>GSMALERTFSIIKPDAVKRNLIGEIYHRIEKAGLQIIAAKMVHLSEEQASGFYAEHEGKPFFEPLKEFMTSGPIMVQVLEGENAIARYRELMGKTNPEEAACGTLRADYALSMRYNSVHGSDSPASAAREIEFFFPESEICPRP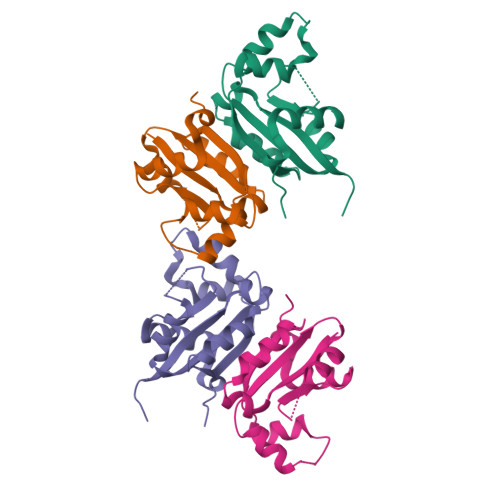[2x]> MQTRTLEIGVGLFLLAGLLALLLLALRVSGLSVGNAGDTYKVY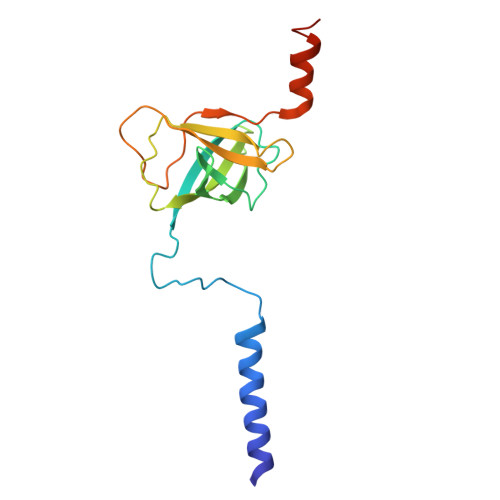AYFDNIAGVTVRGKVTLAGVTIGKVTAVDLDRDSYTGRVTMEINQNVNNLPVDSTASILTAGLLGEKYIGISVGGDEDVLKDGSTIHDTQSALVLEDLIGKFLLNSVNKDEAKK> MPKRIVYNISSDFQLKSLLGEGAYGVVCSATHKPTGEIVAIKKIEPFDKPLFALRTLREIKILKHFKHENIITIFNIQRPDSFENFNEVYIIQELMQTDLHRVISTQMLSDDHIQYFIYQTLRAVKVL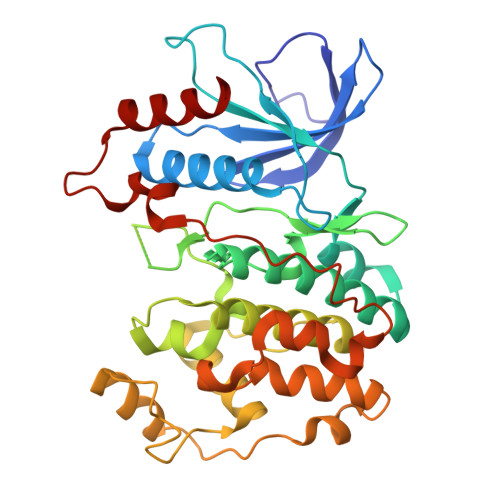HGSNVIHRDLKPSNLLINSNCDLKVCDFGLARIIDESAADNSEPTGQQSGMVEFVATRWYRAPEVMLTSAKYSRAMDVWSCGCILAELFLRRPIFPGRDYRHQLLLIFGIIGTPHSDNDLRCIESPRAREYIKSLPMYPAAPLEKMFPRVNPKGIDLLQRMLVFDPAKRITAKEALEHPYLQTYHDPNDEPEGEPIPPSFFEFDHYKEALTTKDLKKLIWNEIFS> MDYKDDDDKSGSEAEDWTAALLNRGRSRQPLVLGDNCFADLVHNWMELPEEFPAAPAVPGPPGPRSPQREPQRVSHEQFRAALQLVVDPGDPRSYLDNFIKIGEGSTGIVCIATVRSSGKLVAVKKMDLRKQQRRELLFNEV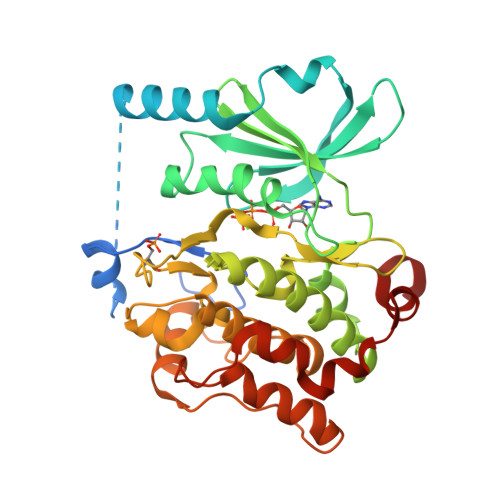VIMRDYQHENVVEMYNSYLVGDELWVVMEFLEGGALTDIVTHTRMNEEQIAAVCLAVLQALSVLHAQGVIHRDIKSDSILLTHDGRVKLSDFGFCAQVSKEVPRRKSLVGTPYWMAPELISRLPYGPEVDIWSLGIMVIEMVDGEPPYFNEPPLKAMKMIRDNLPPRLKNLHKVSPSLKGFLDRLLVRDPAQRATAAELLKHPFLAKAGPPASIVPLMRQNRTR>MPTLSTTNPTLADVAARMTPDGKIDPQIVEMLNETNEILDDMTVIEANGFTEHKTTVRSGLPTGTWRKLNYGVQPEKSRTVQVKDSMGMLETYAEVDKALADLNGNSAAWRLSEDRAFIEGMNQTQATTLFYGDSSIDAEKFMGLTPRFNSLSAENGQNIIDAGGTGSDNASIWLTVWGPNTLHTIYPKGSQAGLQSRDLGEDTLIDAAGGRYQGYRTHYKWDIGLTLRDWRYVVRIANVDVSELTKNASAGADLIDLMTQAVELIPNVGMGRPAFYMPRKIRSFLRRQITNKVAASTLTMEEIAGKKVVAFDGIPCRRTDALLLTEARVV[7x];>[7x]MIIDKLLQVSDGQAVTASAASTDVIDFGQANPNTGMDDRSKMVITVDESADAAGAATVTFSVQDSADNATFADVAATGAIGKANLAAGKQVVIPMPTKLRRYCRVYYTVATGPLTAGKFSAQVVTGIQQNVAYPDSPRIA

Bacteriophage BPP-1 is a short-tailed, dsDNA virus and a member of the Podoviridae family. It infects and kills Bordetella species that cause whooping cough in humans and respiratory diseases in other mammals. It has a T = 7l icosahedral capsid, ∼670 Å in diameter. In this study, we report the three-dimensional (3D) structure of the BPP-1 head at ∼3.5 Å resolution determined by single-particle cryoEM and derived an atomic model.

Arranged on a T = 7 icosahedral shell, MCP and CP each have seven copies or conformers in each asymmetric unit. MCP alone forms a complete icosahedral shell without any noticeable gaps. CP forms dimers bound to the underlying MCP shell at local and icosahedral twofold axes, making the maximum diameter of the BPP-1 (670 Å) bigger than that of the HK97 capsid (659 Å). CP contains two β-sheets each consisting of four anti-parallel strands, and a ∼36-Å long extension (Thr125 to Ala140) with the C-terminus exposed on the external surface. In BPP-1, CP subunits form a dimer through β-sheet augmentation between the F-strands of two CHEF sheets, forming an 8 stranded β-sheet visible on the external surface. Although little sequence identity (CLUSTALW score = 5) was detected between BPP-1 MCP and HK97 gp5 proteins with ClustalW, the overall architecture of the MCP resembles that of HK97 gp5, with an axial (A) domain, a peripheral (P) domain and an extended loop (E-loop). The orders of these three structural elements in BPP-1 and HK97 are N-β-α (‘BPP topology’), N-α-β (‘HK97 topology’), respectively. Moreover, the topology of the Johnson fold in BPP-1 MCP is non-circularly permuted as compared to the previously known topology of the Johnson fold. The P-domain and E-loop of MCP in neighboring capsomers join head to tail to form rings (bright colors), which concatenate to form non-covalent chainmail.> QDWDTFQKKHLTDTKKVKCDVEMKKALFDCKKTNTFIFARPPRVQALCKNIKNNTNVLSRD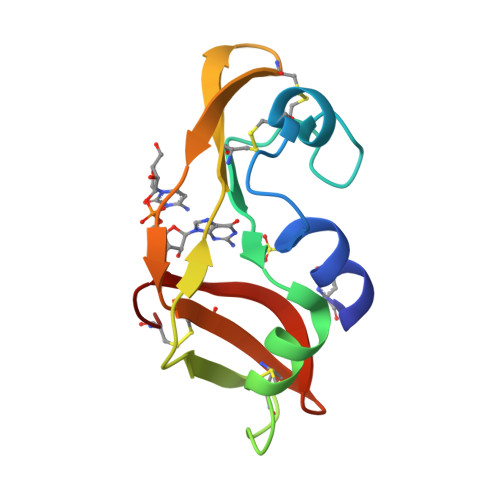VFYLPQCNRKKLPCHYRLDGSTNTICLTCMKELPIHFAGVGKCP>MKNIAILGASGSIGQQAIDVIARHPESFNLISFTVGKNIEFAIEVIEKFKPEIVSVQDEADVERLKPYHSNIVSGRQGLIDVSTYEKNDLVLNALLGSVGLEPTMKAIEAGKNIALANKETLVVAGKLVMTHAKRYGVDILPVDSEHAAIFQCLNGEDMHKIKNVTITASGGSFRELTREQLEHVTVGDALNHPNWSMGNKITIDSATMMNKGFEVIEAKWLFDLKIDQIKTILHKESIIHSLVEFVDTSVMAQLGTPDMRMPIQYAFTYPERIEHRAPSLDLVQVAQLHFQEMDLDRYRCLKFAYDALRIGGSMPVVLNAVNEVAVAKFLNHEITFLEI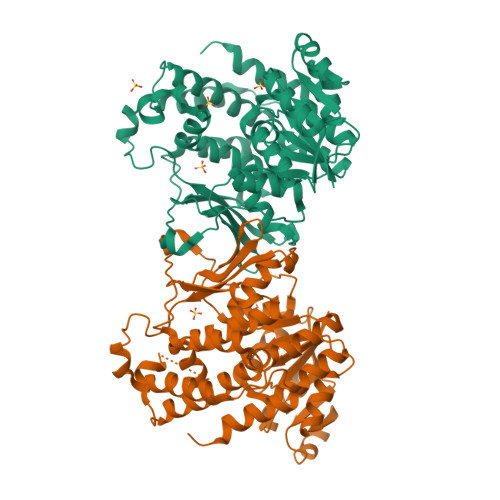EHMIEREMSAHEVIPDPSLEEILEIDHYYKTKSYEV[2x]>STTGIIMENVTAFWEEGFGELLEKVQQSNGDRKHSSDENNVSFSHLCLVGNPVLKNINLNIEKGEMLAITGSTGSGKTSLLMLILGELEASEGIIKHSGRVSFCSQFSWIMPGTIKENIIRGVSYDEYRYKSVVKACQLQQDITKFAEQDNTVLGEGGVTLSGGQRARISLARAVYKDADLYLLDSPFGYLDVFTEEQVFESCVCKLMANKTR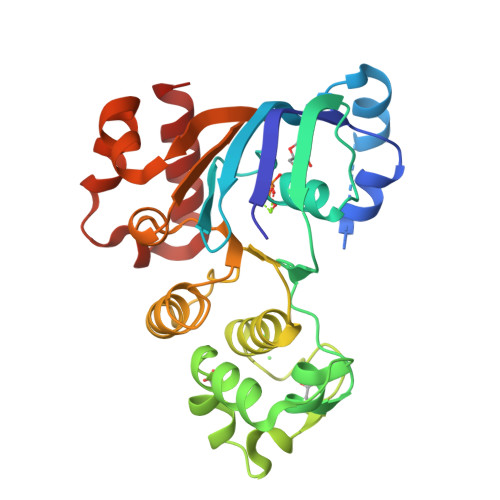ILVTSKMEHLRKADKILILHQGSSYFYGTFSELQSLRPDFSSKLMGYDTFDQFTEERRSSILTETLRRFS[2x]> GILAEAHGTRPDLTDQPLPDADHTWYTDGSSLLQEGQRKAGAAVTTETEVIWAKALPAGTSAQRAELIALTQALKMAEGKKLNVYTDSRYAFATAH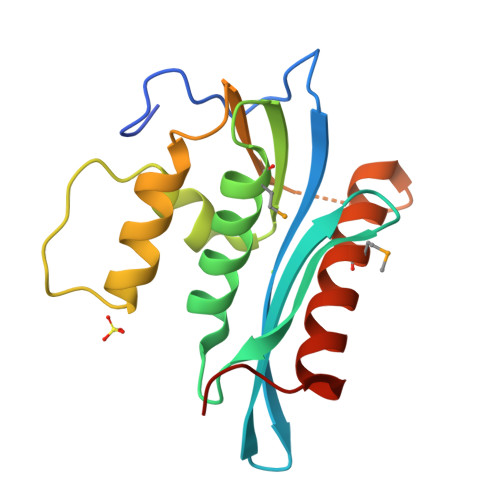LTSEGKEIKNKDEILALLKALFLPKRLSIIHCPGHQKGHSAEARGNRMADQAARKAAITETPDTSTLL>[5x]MSEYIRVTEDENDEP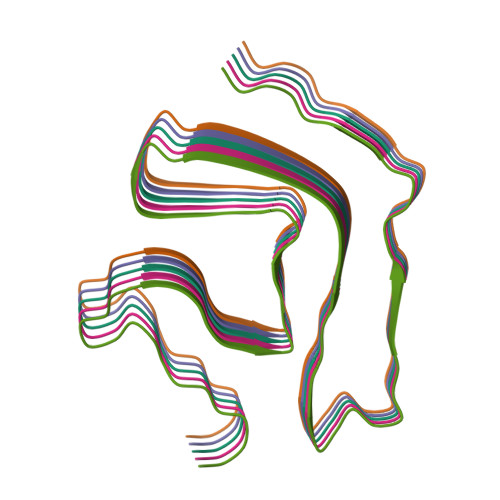IEIPSEDDGTVLLSTVTAQFPGACGLRYRNPVSQCMRGVRLVEGILHAPDAGWGNLVYVVNYPKDNKRKMDETDASSAVKVKRAVQKTSDLIVLGLPWKTTEQDLKEYFSTFGEVLMVQVKKDLKTGHSKGFGFVRFTEYETQVKVMSQRHMIDGRWCDCKLPNSKQSQDEPLRSRKVFVGRCTEDMTEDELREFFSQYGDVMDVFIPKPFRAFAFVTFADDQIAQSLCGEDLIIKGISVHISNAEPKHNSNRQLERSGRFGGNPGGFGNQGGFGNSRGGGAGLGNNQGSNMGGGMNFGAFSINPAMMAAAQAALQSSWGMMGMLASQQNQSGPSGNNQNQGNMQREPNQAFGSGNNSYSGSNSGAAIGWGSASNAGSGSGFNGGFGSSMDSKSSGWGM>[6x]TLPKRVKIVEVGPRDGLQNEKNIVSTPVKIKLIDMLSE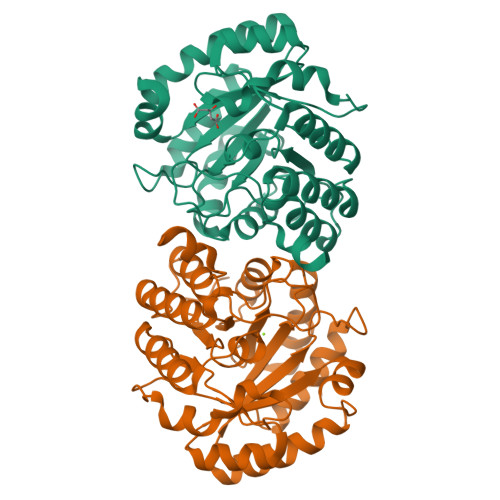AGLSVIETTSFVSPKWVPQMGDHTEVLKGIQKFPGINYPVLTPNLKGFEAAVAAGAKEVVIFGAASELFTKKNINCSIEESFQRFDAILKAAQSANISVRGYVSCALGCPYEGKISPAKVAEVTKKFYSMGCYEISLGDTIGVGTPGIMKDMLSAVMQEVPLAALAVHCHDTYGQALANTLMALQMGVSVVDSSVAGLGGCPYAQGASGNLATEDLVYMLEGLGIHTGVNLQKLLEAGNFICQALNRKTSSKVAQATCKL> AGITGTWYAQLGDTFIVTAGADGALTGTYEAAVGNAESRYVLTGRYDSAPATDGSGTALGWTVAWKNNYRNAHSATTWSGQYVGGAEARINTQWLLTSGTTEANAWKSTLVGH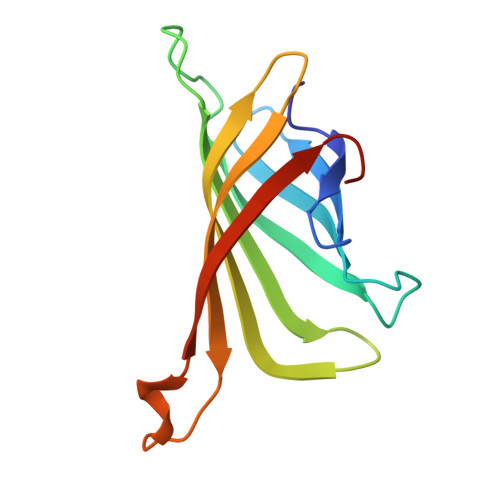DTFTKVKPSAAS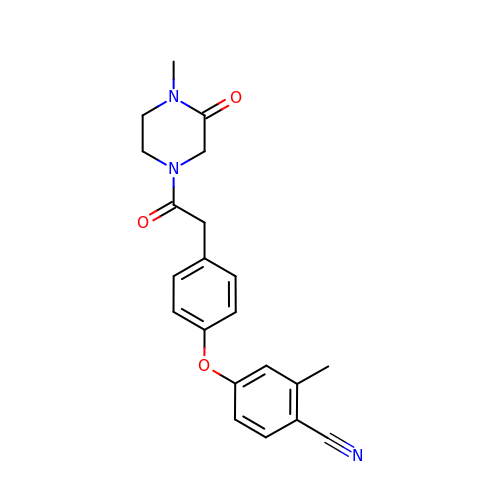2-methyl-4-{4-[2-(4-methyl-3-oxopiperazin-1-yl)-2-oxoethyl]phenoxy}benzonitrile | C21 H21 N3 O3 | WFOOODRZHBDNTB-UHFFFAOYSA-N> AAAUUGAAGAGUUUGAUCAUGGCUCAGAUUGAACGCUGGCGGCAGGCCUAACACAUGCAAGUCGAACGGUAACAGGAAGAAGCUUGCUUCUUUGCUGACGAGUGGCGGACGGGUGAGUAAUGUCUGGGAAACUGCCUGAUGGAGGGGGAUAACUACUGGAAACGGUAGCUAAUACCGCAUAACGUCGCAAGACCAAAGAGGGGGACCUUCGGGCCUCUUGCCAUCGGAUGUGCCCAGAUGGGAUUAGCUAGUAGGUGGGGUAACGGCUCACCUAGGCGACGAUCCCUAGCUGGUCUGAGAGGAUGACCAGCCACACUGGAACUGAGACACGGUCCAGACUCCUACGGGAGGCAGCAGUGGGGAAUAUUGCACAAUGGGCGCAAGCCUGAUGCAGCCAUGCCGCGUGUAUGAAGAAGGCCUUCGGGUUGUAAAGUACUUUCAGCGGGGAGGAAGGGAGUAAAGUUAAUACCUUUGCUCAUUGACGUUACCCGCAGAAGAAGCACCGGCUAACUCCGUGCCAGCAGCCGCGGUAAUACGGAGGGUGCAAGCGUUAAUCGGAAUUACUGGGCGUAAAGCGCACGCAGGCGGUUUGUUAAGUCAGAUGUGAAAUCCCCGGGCUCAACCUGGGAACUGCAUCUGAUACUGGCAAGCUUGAGUCUCGUAGAGGGGGGUAGAAUUCCAGGUGUAGCGGUGAAAUGCGUAGAGAUCUGGAGGAAUACCGGUGGCGAAGGCGGCCCCCUGGACGAAGACUGACGCUCAGGUGCGAAAGCGUGGGGAGCAAACAGGAUUAGAUACCCUGGUAGUCCACGCCGUAAACGAUGUCGACUUGGAGGUUGUGCCCUUGAGGCGUGGCUUCCGGAGCUAACGCGUUAAGUCGACCGCCUGGGGAGUACGGCCGCAAGGUUAAAACUCAAAUGAAUUGACGGGGGCCCGCACAAGCGGUGGAGCAUGUGGUUUAAUUCGAUGCAACGCGAAGAACCUUACCUGGUCUUGACAUCCACGGAAGUUUUCAGAGAUGAGAAUGUGCCUUCGGGAACCGUGAGACAGGUGCUGCAUGGCUGUCGUCAGCUCGUGUUGUGAAAUGUUGGGUUAAGUCCCGCAACGAGCGCAACCCUUAUCCUUUGUUGCCAGCGGUCCGGCCGGGAACUCAAAGGAGACUGCCAGUGAUAAACUGGAGGAAGGUGGGGAUGACGUCAAGUCAUCAUGGCCCUUACGACCAGGGCUACACACGUGCUACAAUGGCGCAUACAAAGAGAAGCGACCUCGCGAGAGCAAGCGGACCUCAUAAAGUGCGUCGUAGUCCGGAUUGGAGUCUGCAACUCGACUCCAUGAAGUCGGAAUCGCUAGUAAUCGUGGAUCAGAAUGCCACGGUGAAUACGUUCCCGGGCCUUGUACACACCGCCCGUCACACCAUGGGAGUGGGUUGCAAAAGAAGUAGGUAGCUUAACCUUCGGGAGGGCGCUUACCACUUUGUGAUUCAUGACUGGGGUGAAGUCGUAACAAGGUAACCGUAGGGGAACCUGCGGUUGGAUCACCUCCUUA;> GGUUAAGCGACUAAGCGUACACGGUGGAUGCCCUGGCAGUCAGAGGCGAUGAAGGACGUGCUAAUCUGCGAUAAGCGUCGGUAAGGUGAUAUGAACCGUUAUAACCGGCGAUUUCCGAAUGGGGAAACCCAGUGUGUUUCGACACACUAUCAUUAACUGAAUCCAUAGGUUAAUGAGGCGAACCGGGGGAACUGAAACAUCUAAGUACCCCGAGGAAAAGAAAUCAACCGAGAUUCCCC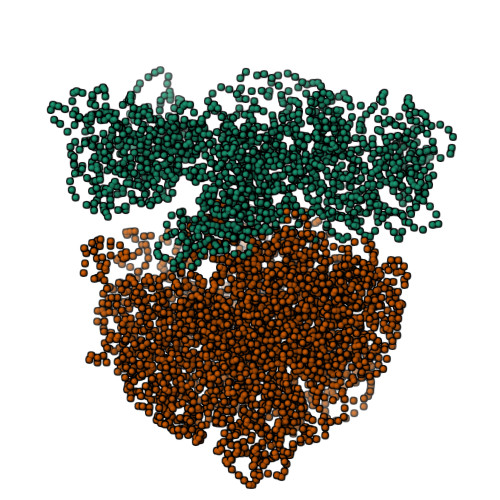CAGUAGCGGCGAGCGAACGGGGAGCAGCCCAGAGCCUGAAUCAGUGUGUGUGUUAGUGGAAGCGUCUGGAAAGGCGCGCGAUACAGGGUGACAGCCCCGUACACAAAAAUGCACAUGCUGUGAGCUCGAUGAGUAGGGCGGGACACGUGGUAUCCUGUCUGAAUAUGGGGGGACCAUCCUCCAAGGCUAAAUACUCCUGACUGACCGAUAGUGAACCAGUACCGUGAGGGAAAGGCGAAAAGAACCCCGGCGAGGGGAGUGAAAAAGAACCUGAAACCGUGUACGUACAAGCAGUGGGAGCACGCUUAGGCGUGUGACUGCGUACCUUUUGUAUAAUGGGUCAGCGACUUAUAUUCUGUAGCAAGGUUAACCGAAUAGGGGAGCCGAAGGGAAACCGAGUCUUAACUGGGCGUUAAGUUGCAGGGUAUAGACCCGAAACCCGGUGAUCUAGCCAUGGGCAGGUUGAAGGUUGGGUAACACUAACUGGAGGACCGAACCGACUAAUGUUGAAAAAUUAGCGGAUGACUUGUGGCUGGGGGUGAAAGGCCAAUCAAACCGGGAGAUAGCUGGUUCUCCCCGAAAGCUAUUUAGGUAGCGCCUCGUGAAUUCAUCUCCGGGGGUAGAGCACUGUUUCGGCAAGGGGGUCAUCCCGACUUACCAACCCGAUGCAAACUGCGAAUACCGGAGAAUGUUAUCACGGGAGACACACGGCGGGUGCUAACGUCCGUCGUGAAGAGGGAAACAACCCAGACCGCCAGCUAAGGUCCCAAAGUCAUGGUUAAGUGGGAAACGAUGUGGGAAGGCCCAGACAGCCAGGAUGUUGGCUUAGAAGCAGCCAUCAUUUAAAGAAAGCGUAAUAGCUCACUGGUCGAGUCGGCCUGCGCGGAAGAUGUAACGGGGCUAAACCAUGCACCGAAGCUGCGGCAGCGACGCUUAUGCGUUGUUGGGUAGGGGAGCGUUCUGUAAGCCUGCGAAGGUGUGCUGUGAGGCAUGCUGGAGGUAUCAGAAGUGCGAAUGCUGACAUAAGUAACGAUAAAGCGGGUGAAAAGCCCGCUCGCCGGAAGACCAAGGGUUCCUGUCCAACGUUAAUCGGGGCAGGGUGAGUCGACCCCUAAGGCGAGGCCGAAAGGCGUAGUCGAUGGGAAACAGGUUAAUAUUCCUGUACUUGGUGUUACUGCGAAGGGGGGACGGAGAAGGCUAUGUUGGCCGGGCGACGGUUGUCCCGGUUUAAGCGUGUAGGCUGGUUUUCCAGGCAAAUCCGGAAAAUCAAGGCUGAGGCGUGAUGACGAGGCACUACGGUGCUGAAGCAACAAAUGCCCUGCUUCCAGGAAAAGCCUCUAAGCAUCAGGUAACAUCAAAUCGUACCCCAAACCGACACAGGUGGUCAGGUAGAGAAUACCAAGGCGCUUGAGAGAACUCGGGUGAAGGAACUAGGCAAAAUGGUGCCGUAACUUCGGGAGAAGGCACGCUGAUAUGUAGGUGAGGUCCCUCGCGGAUGGAGCUGAAAUCAGUCGAAGAUACCAGCUGGCUGCAACUGUUUAUUAAAAACACAGCACUGUGCAAACACGAAAGUGGACGUAUACGGUGUGACGCCUGCCCGGUGCCGGAAGGUUAAUUGAUGGGGUUAGCGCAAGCGAAGCUCUUGAUCGAAGCCCCGGUAAACGGCGGCCGUAACUAUAACGGUCCUAAGGUAGCGAAAUUCCUUGUCGGGUAAGUUCCGACCUGCACGAAUGGCGUAAUGAUGGCCAGGCUGUCUCCACCCGAGACUCAGUGAAAUUGAACUCGCUGUGAAGAUGCAGUGUACCCGCGGCAAGACGGAAAGACCCCGUGAACCUUUACUAUAGCUUGACACUGAACAUUGAGCCUUGAUGUGUAGGAUAGGUGGGAGGCUUUGAAGUGUGGACGCCAGUCUGCAUGGAGCCGACCUUGAAAUACCACCCUUUAAUGUUUGAUGUUCUAACGUUGACCCGUAAUCCGGGUUGCGGACAGUGUCUGGUGGGUAGUUUGACUGGGGCGGUCUCCUCCUAAAGAGUAACGGAGGAGCACGAAGGUUGGCUAAUCCUGGUCGGACAUCAGGAGGUUAGUGCAAUGGCAUAAGCCAGCUUGACUGCGAGCGUGACGGCGCGAGCAGGUGCGAAAGCAGGUCAUAGUGAUCCGGUGGUUCUGAAUGGAAGGGCCAUCGCUCAACGGAUAAAAGGUACUCCGGGGAUAACAGGCUGAUACCGCCCAAGAGUUCAUAUCGACGGCGGUGUUUGGCACCUCGAUGUCGGCUCAUCACAUCCUGGGGCUGAAGUAGGUCCCAAGGGUAUGGCUGUUCGCCAUUUAAAGUGGUACGCGAGCUGGGUUUAGAACGUCGUGAGACAGUUCGGUCCCUAUCUGCCGUGGGCGCUGGAGAACUGAGGGGGGCUGCUCCUAGUACGAGAGGACCGGAGUGGACGCAUCACUGGUGUUCGGGUUGUCAUGCCAAUGGCACUGCCCGGUAGCUAAAUGCGGAAGAGAUAAGUGCUGAAAGCAUCUAAGCACGAAACUUGCCCCGAGAUGAGUUCUCCCUGACCCUUUAAGGGUCCUGAAGGAACGUUGAAGACGACGACGUUGAUAGGCCGGGUGUGUAAGCGCAGCGAUGCGUUGAGCUAACCGGUACUAAUGAACCGUGAGGCUUAACCUU>MGKFVEKLEKAIKGYTFDDVLLIPQATEVEPKDVDVSTRITPNVKLNIPILSAAMDTVTEWEMAVAMAREGGLGVIHRNMGIEEQVEQVKRVKRAERLIVEDVITIAPDETVDFALFLMEKHGIDGLPVVEDEKVVGIITKKDIAAREGKLVKELMTKEVITVPESIEVEEALKIMIENRIDRLPVVDERGKLVGLITMSDLVARKKYKNAVRDENGELLVAAAVSPFDIKRAIELDKAGVDVIVVDTAHAHNLKAIKSMKEMRQKVDADFIVGNIANPKAVDDLTFADAVKVGIGPGSICTTRIVAGVGVPQITAVAMVADRAQEYGLYVIAD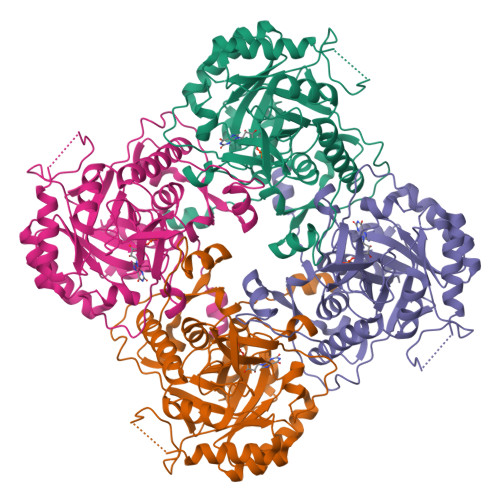GGIRYSGDIVKAIAAGADAVMLGNLLAGTKEAPGKEVIINGRKYKQYRGMGSLGAMMKGGAERYYQGGYMKTRKFVPEGVEGVVPYRGTVSEVLYQLVGGLKAGMGYVGARNIRELKEKGEFVIITHAGIKESHPHDIIITNEAPNYPLEKF[2x]> MTIKNFTFFSPNSTEFPVGSNNDGKLYMMLTGMDYRTIRRKDWSSPLNTALNVQYTNTSIIAGGRYFELLNETVALKGDSVNYIHANIDLTQTANPVSLSAETANNSNGVDINNGSGVLKVCFDIVTTSGTGVTSTKPIVQTSTLDSISVNDMTVSGSIDVPVQTLTVEAGNGLQLQLTKKNNDLVIVRFFGSVSNIQKGWNMSGTWVDRPFRPAAVQSLVGHFA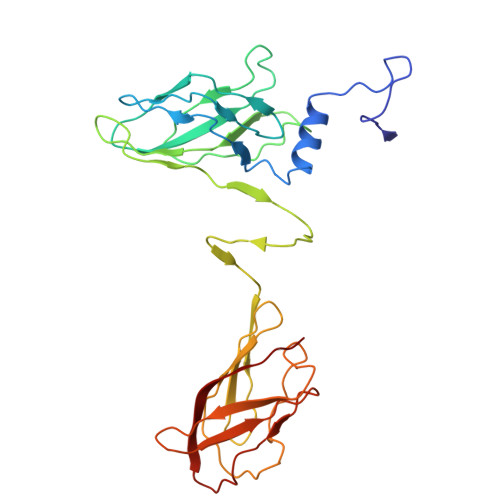GRDTSFHIDINPNGSITWWGANIDKTPIATRGNGSYFIK>TSLKQAYAQGFLLGTAVNADIVSGKDAASAALVACHFNAVTAENVMKAEVVAPRRGVQDFSAADAFVAYAQRDRQFVVGHTLVWHNQTPEWFFTTADGRPNTPAQQLERMRAHIAAVAGRYTGKVQAWDVVNEIIDEDGSYRSTNWVQRVGDGDT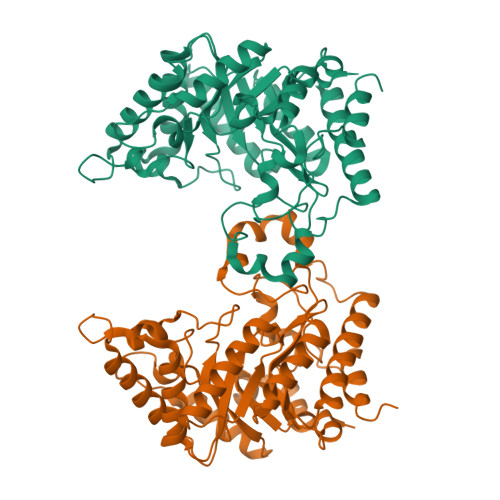VVRNAFAFAQRYAPDAQLYYNDFNAWRPAKREGIVRMVKMLQQAGVRIDGVGMQGHWGLNYPSLRDIEDAIDAYAALGVKVMITELDIDVLPLTKEGQIIGTGMAHKQFQLPEFKRFLDPYRDGLPADVQAQLRDRYAELFALFWRKRDKIARVSVWGVSDDMSWKNDYPVPGRTNYPLLFDRNHQPKPALDAVVAVPSAT[6x]> MPPGVDCPMEFWTKEENQSVVVDFLLPTGVYLNFPVSRNANLSTIKQLLWHRAQYEPLFHMLSGPEAYVFTCINQTAEQQELEDEQRRLCDVQPFLPVLRLVAREGDRVKKLINSQISLLIGKGLHEFDSLCDPEVNDFRAKMCQFCEEAAARRQQLGWEAWLQYSFPLQLEPSAQTWGPGTLRLPNRALLVNVKFEGSEESFTFQVSTKDVPLALMACALRKKATVFRQPLVEQPEDYTLQVNGRHEYLYGSYPLCQFQYICSCLHSGLTPHLTMVHSSSILAMRDEQSNPAPQVQKPRAKPPPIPAKKPSSVSLWSLEQPFRIELIQGSKVNADERMKLVVQAGLFHGNEMLCKTVSSSEVSVCSEPVWKQRLEFDINICDLPRMARLCFALYAVIEKAKKARSTKKKSKKADCPIAWANLMLFDYKDQLKTGERCLYMWPSVPDEKGELLNPTGTVRSNPNTDSAAALLICLPEVAPHPVYYPALEKILELGRHSECVHVTEEEQLQLREILERRGSGELYEHEKDLVWKLRHEVQEHFPEALARLLLVTKWNKHEDVAQMLYLLCSWPELPVLSALELLDFSFPDCHVGSFAIKSLRKLTDDELFQYLLQLVQVLKYESYLDCELTKFLLDRALANRKIGHFLFWHLRSEMHVPSVALRFGLILEAYCRGSTHHMKVLMKQGEALSKLKALNDFVKLSSQ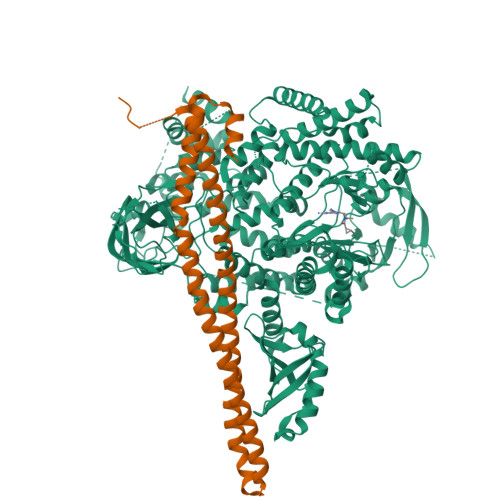KTPKPQTKELMHLCMRQEAYLEALSHLQSPLDPSTLLAEVCVEQCTFMDSKMKPLWIMYSNEEAGSGGSVGIIFKNGDDLRQDMLTLQMIQLMDVLWKQEGLDLRMTPYGCLPTGDRTGLIEVVLRSDTIANIQLNKSNMAATAAFNKDALLNWLKSKNPGEALDRAIEEFTLSCAGYCVATYVLGIGDRHSDNIMIRESGQLFHIDFGHFLGNFKTKFGINRERVPFILTYDFVHVIQQGKTNNSEKFERFRGYCERAYTILRRHGLLFLHLFALMRAAGLPELSCSKDIQYLKDSLALGKTEEEALKHFRVKFNEALRESWKTKVNWLAHNVSKDNRQ;> MYQQDQVVKEDNIEAVGKKLHEYNTQFQEKSREYDRLYEDYTRTSQEIQMKRTAIEAFNETIKIFEEQCQTQERYSKEYIEKFKREGNETEIQRIMHNYEKLKSRISEIVDSRRRLEEDLKKQAAEYREIDKRMNSIKPDLIQLRKTRDQYLMWLTQKGVRQKKLNEWLGNSRACSLEACGTKLVEKY>[84x]MSGFGGGSSGAGSLTQLLATGSMDAALTQNATRTFWKSSYQKHSLFALESINQPFTTQVQFGAESHITVNRQGDLLSWMYLKIVLPGLKVQNQADTVQPTQQSFASLDNDVAAQADVSHVLPYIEGAYTEASLNTKEQLIAEAKNSYEAAKYNAAPLPVAAQMQSTEMPDFDYAYWTEAIGFHLIKRAEFKVGGATIDTIWSELLFAMEELMGRAGRRLTETIGRTLRRPTELMKASRQEQILYVPLPWYFTKHPSLAFPLVAATYHNIQLWVQWAQLNSCIIKSRSNLVVLHAERNVPISDDHLRASLECTYVHLEAAERDALTANAGTQLIVQHQAHLQQVSSNNVTARLNFNFPVLEFYYFLRRKANKDAGDHFNFSGIGGRDPVVSAELLFNNTARVTQKPAVWWRAVQALQFHSSAPLTNIYSYSFSLSPEDPITPSGSANFSRLDSVELALTLQDDFGAAHDANSELFVFARSYNILKFTNGLAGLLYSN;> MPSIAFSGISTKPGELEFHVPSVLSKHNRAGLLKSIDFPYSQRTIESSWNKLHYMESIRITPESRSVSVLLTDKESGDRVEMLAMVPLTTNKIIEISTATTDGTIILVTEEPHGFFAPGCFGKEVRNVISSYKSIFPHGTPPFILIHGSNGSVQVDPALFEYNDEYSVKIKYTAIRTEFKLFGKGDHGWMVTPEFPTISMLCQVITNAMNSAIIFNHDDPAARTRMYPGTCSNTHVIESVSGDSLAKALLGYDGVYAGWEEITIPAGMYCYGELDLSKMIAAKMNRWHIDRESSIIFRGVSGYTWNVTLPSGNYGTPEKLAHCIQHMMNMTAKNRKNPYCVRFTLNEGSSHRGKFVFVAAEPFDLLFGDDESIDPSILGFEPVDHIGRNSYMSENDLGAPLMKPNCNVYDVDEIPGTHQIRIGRRTRLAVDGKIRGYSGGTLRLNTVNRTTGAPKCHGMNKGDVVTLTTVMPAPDGATGTKREGFTFRAKNKIMGVVVADENENPDASSLHVSVPSMSWTLGIGSYITIDSQAAPISVALFDPGKNQFFRDSIGASRLGFSNGVSTGQHGVVVSQCAVNLEPRTVDVSFIEGSMTSASTEMYNQNGKSLITQVPSDRSSGPVPQGMVRFNNALQQFKLEFTNPDGSPYHFNHASLSLLMEFDD

The population density of E. huxleyi is restricted by Nucleocytoviricota viruses, including E. huxleyi virus 201 (EhV-201). Here, we show that the dsDNA genome inside the EhV-201 virion is protected by an inner membrane, capsid, and outer membrane. Virions of coccolithoviruses are unique within the family Phycodnaviridae because they contain not only a membrane inside the capsid but also an additional membrane wrapped around the outer capsid surface, similar to the African swine fever virus from the family Asfaviridae. EhV-201 virions infect E. huxleyi by using fivefold vertices to bind to and fuse the virus’ inner membrane with the cell plasma membrane.

(E) Composite map of EhV-201 virion. The surface of the virion is covered with the outer membrane (gray) with central (red) and peripheral (light blue) vertex proteins and dimers of ridge proteins (light yellow and gray ripples on the virion surface). Penton proteins are shown in purple whereas major capsid proteins are in various other colors. (F) AlphaFold2-predicted structure of EhV-201 major capsid protein with double jelly roll fold. The jellyroll cores J1 and J2 are each composed of two β sheets named according to the convention BIDG and CHEF. The EhV-201 virion contains 60 copies of each central and peripheral vertex protein and at least 1320 copies of ridge protein. The forming capsids have straight edges and angular vertices, which indicate that they assemble according to the rules of quasi-icosahedral symmetry as is the case for NCVs with isometric capsids.>[5x]SNAMIIRPEQHWFLRLFDWHGSVLSKIIFRLLLNVLMSIIAIISYQWYEQLGIHLTVAPFSLLGIAIAIFLGFRNSASYSRFVEARNLWGTVLIAERTLVRQLRNILPAEHDAHRR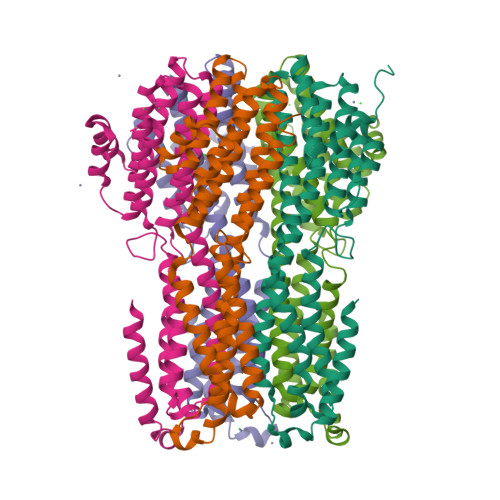IVSYLVAFSWSLKHQLRKTDPTADLRRLLPEERVTEILASSMPTNRILLLAGNEIGQLREAGKLSDITYGLMDNKLDELAHVLGGCERLATTPVPFAYTLILQRTVYLFCTLLPFALVGDLHYMTPFVSVFISYTFLSWDSLAEELEDAFGTAANDLPLNAMCNTIERNLLDMTGQHPLPE>[2x]GPGGSGGMKPQIRNMVEPMDPRTFVSNFNNRPILSGLDTVWLCCEVKTKDPSGPPLDAKIFQGKVYPKAKYHPEMRFLRWFHKWRQLHHDQEYKVTWYVSWSPCTRCANSVATFLAKDPKVTLTIFVARLYYFWDPDYQQALRILAEAGATMKIMNYNEFQDCWNKFVDGRGKPFKPWNNLPKHYTLLQATLGE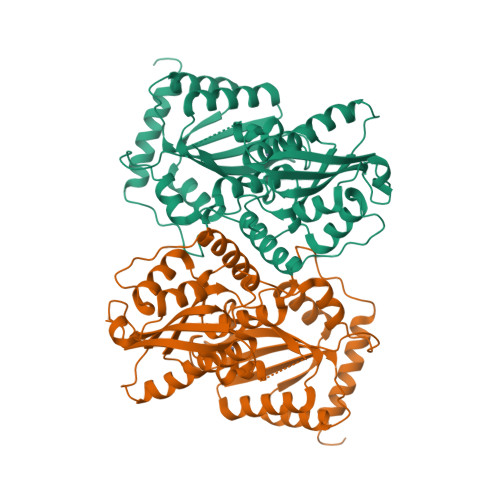LLRHLMDPGTFTSNFNNKPWVSGQHETYLCYKVERLHNDTWVPLNQHRGFLRNQAPNIHGFPKGRHAQLCFLDLIPFWKLDGQQYRVTCFTSWSPCFSCAQEMAKFISNNEHVSLCIFAARIYDDQGRYQEGLRTLHRDGAKIAMMNYSEFEYCWDTFVDRQGRPFQPWDGLDEHSQALSGRLRAILQNQGN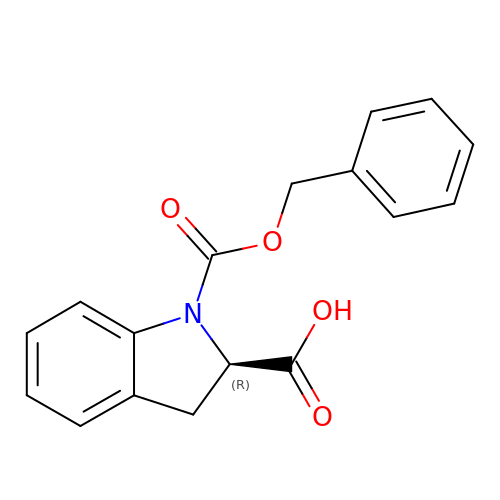(2R)-1-[(benzyloxy)carbonyl]-2,3-dihydro-1H-indole-2-carboxylic acid | C17 H15 N O4 | BSOYWTITVKXHLM-OAHLLOKOSA-N DgkA is a homo-trimeric kinase involved in phospholipid metabolism in Gram negative bacteria. The smallest known kinase, it consists of four helices, three of which are either fully or partly membrane embedded while the fourth resides at the membrane surface. DgkA is a promiscuous enzyme and, in addition to using diacylglycerol as a substrate, it can also phosphorylate the mesophase forming monoolein. Having long served as a model for studies of membrane protein folding, assembly and stability, DgkA was chosen as the test protein.

The structure of a wild-type and a fully functional, thermostable variant was determined recently to 3.7 Å and 2.05 Å, respectively, using crystals grown in meso. The two DgkA constructs gave almost identical results in this study. The renaturation hypothesis was tested by mixing monoolein with a solution of denatured DgkA* dissolved in acidic urea and then bathing the spontaneously-assembled mesophase in denaturant-free buffer. Thus, the simple process of mesophase formation and bathing with excess denaturant-free solvent facilitated a transformation from unfolded kinase monomers in denaturant solution to membrane integral, refolded and properly assembled trimers with full enzymatic activity. Likewise, the refolded wild-type DgkA* was crystallized in meso using 9.9 MAG or 7.8 MAG as host lipids. Crystals in 9.9 MAG diffracted to 4 Å. A complete data set to 3.8 Å was obtained with crystals grown in 7.8 MAG and was used for structure determination. The structure of the refolded wild-type DgkA* is virtually identical (RMSD, 0.419 Å) to the 3.7 Å structure recorded for the untreated, reference wild-type enzyme.

>GHHHHHHELANNTTGFTRIIKAAGYSWKGLRAAWINEAAFRQEGVAVLLAVVIACWLDVDAITRVLLISSVMLVMIVEILNSAIEAVVDRIGSEYHELSGRAKDMGSAAVLIAIIVAVITWCILLWSHFG[3x]>HHHHHHASMDKNIIIGAMTALITPFKNGKVDEQSYARLIKRQIENGIDAVVPV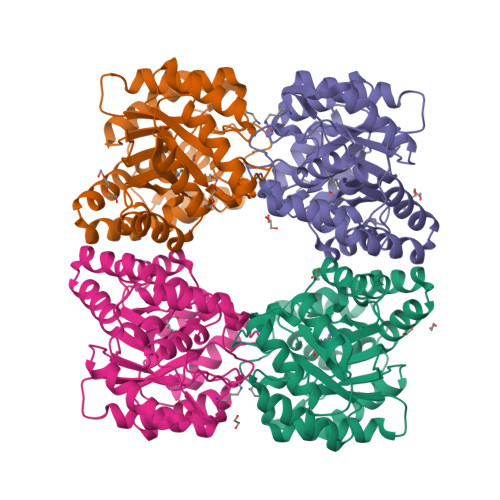GTTGESATLTHEEHRTCIEIAVETCKGTKVKVLAGAGSNATHEAVGLAKFAKEHGADGILSVAPFYNKPTQQGLYEHYKAIAQSVDIPVLLYNVPGRTGCEISTDTIIKLFRDCENIYGVKEASGNIDKCVDLLAHEPRMMLISGEDAINYPILSNGGKGVISVTSNLLPDMISALTHFALDENYKEAKKINDELYNINKILFCESNPIPIKTAMYLAGLIESLEFRLPLCSPSKENFAKIEEVMKKYKIKGF[8x]>[2x]MRALPDVRDGLKPVHRRVLFAMDVLGNDWNKAYKKSARVVGDVIGKYH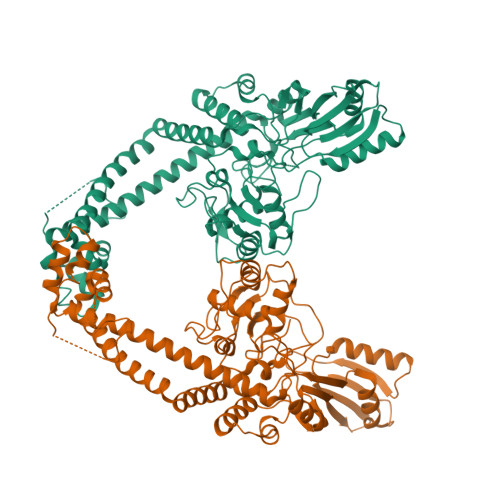PHGDTAVYDTIVRMAQPFSLRYMLVDGQGNFGSVDGDSAAAMRYTEIRMSKIAHSILADLDKETVDFVPNYDGTEHIPAVMPTRVPNLLVNGTSGIAVGMATNIPPHNLTEVINACLALIDNSELTFEEILEHIPGPDFPTAGIISGRAGIEEAYRTGRGKIKIRARASIDVHETTGKETIIVHELPYQVNKARLIEKMAELVKDKRLEGISALRDESDKDGMRMVIEIKRGEVGEVVLNNLYKLTQMQVSFGLNMVALTNGQPKIFNIKEMLEAFVLHRREVVTRRTIFELRKARDRAHILEGLSIALANIDPIIEMIKNSNNRKESEEKLISQGWELGNVANMLSEAGNDAARPEWLEPEYGIRDGLYYLTAEQAKAIVDLQLYKLSGMEHDKILSEYKALLDLIAELMHILATPARLMEVICEELVAIRDEFGDERRTEITLEHHHHHH> PLPTPVGMEIMPPQPPLPPDSSSQDCDPTASLRPFATKAEADAAVADIRARGRLIVGLDIGSNLFSFRDPITGEITGFDVDIAGEV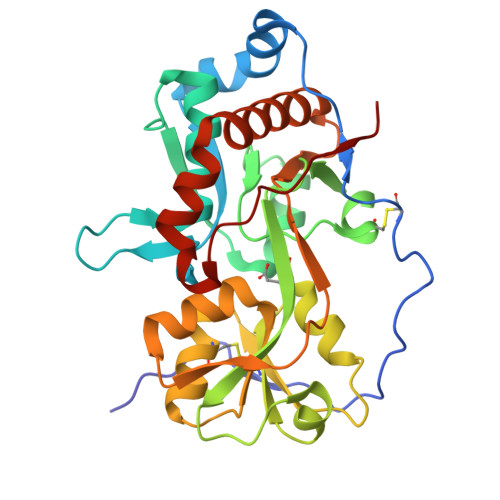ARDIFGVPSHVEYRILSAAERVTALQKSQVDIVVKTMSITCERRKLVNFSTVYLDANQRILAPRDSPITKVSDLSGKRVCVARGTTSLRRIREIAPPPVIVSVVNWADCLVALQQREIDAVSTDDTILAGLVEEDPYLHIVGPDMADQPYGVGINLDNTGLVRFVNGTLERIRNDGTWNTLYRKWLTVLGPAPAPPTPRYVD>[2x]MEKRMSTQQRAAGNACPTAAFSFDPARLAQRRRWAGAFAALCGLALSPSALLAEEHSQHQDHAVELAPSVVTGVAQSSPLTIVTNPKEPRQPVPASDGADYLKTIPGFAVIRNGGSNGDPVLRGMFGSRLNILTNGGMMLGAAPNRMDAPTSYISPETYDKLTVIKGPQTVLWGPGASAGTILFEREPERFGELGSRVNASLLAGSNGRFDKVLDAAAGNRLGYLRFTGNHAQSDDYEDGAGNTVPSRWKKWNGDVAVGWTPDEDTLIELTAGKGDGEARYAGRGMDGSQFKRESLGLRFVKSNVSDVLEKVEAQVYYNYADHIMDNFRLRTPDPSSMMPMPMASQVDRRTLGGRLAATWRWDDFKLVTGVDAMRNEHRARGSKYDMMTDYYTDADQFPWSKDAVFHNYGAFGELTWFAAERDRLIGGLRLDRASVKDYRQTLKSGHMGHAMANPTANDTRADTLPSGFVRYEHDLADSPTTLYAGLGHAERFPDYWELFSPKRGPNGSVNAFDKIKPEKTTQLDFGLQYNGDKLQAWASGYVGVVQDFILFSYREGMMGSSTQATNVDARIMGGELGASYQLTGNWKTDASLAYAWGKNSSDDRALPQIPPLEARFGLTYEEGDWSAGSLWRVVAPQNRIARDQGNVVGKDFDKSAGFGVFSLNGAYRVTRNVKLSAGVDNLFDKDYTEHLNKAGDAGFGFSANETVPEPGRTFWTKVDFSF

Here, we show that Pseudomonas aeruginosa OprC is an outer membrane, TonB-dependent transporter that is conserved in many Proteobacteria and which mediates acquisition of both reduced and oxidised ionic copper via an unprecedented CxxxM-HxM metal binding site. As indicated by the successful structure solution, OprC contains a single bound copper and shows the typical fold of a TBDT, with a large 22-stranded β-barrel occluded by an N-terminal approximately 15 kDa plug domain that, like in other TBDTs, completely occludes the lumen of the barrel. The copper binding site comprises residues Cys143 and Met147 in the plug domain and His323 and Met325 in the barrel wall. The CxxxM-HxM configuration, which coordinates the copper in a tetrahedral manner, is highly unusual and has, to our knowledge, not been observed before in copper homeostasis proteins.

Since Cu(II) prefers histidine nitrogen as ligands and Cu(II) binding sites often contain one or more His residues, we also cocrystallised the H323A mutant with Cu(II) and Ag(I). With Ag(I), 2 clear anomalous peaks are observed, suggesting that the H323A mutant can still bind Cu(I) at the principal site and at the methionine track. All 4 residues in the OprC binding site contribute to copper binding, but not to the same extent and, in some cases, not equally for both copper redox states. By contrast, removal of His323 still allows Cu(II) and Cu(I) binding.> MGHHHHHHHHHHSSGHIEGRHMRVGYVSTNYSLGCKADKTIKLSSLSEERVLKVSSSNLLCLKNILEWNLKHEILFFRISSNTIPLASHPKFHVNWKDKLSHILGDIGDFIKENSIRISMHPGQYVVLNSVREEVVRSSIMELKYHADLLDSMGIEGKIQIHVGSSMNGKEESLNRFIENFRKLPSNISKRLVIENDDKVFSVKDCLWISERTGIPVIFD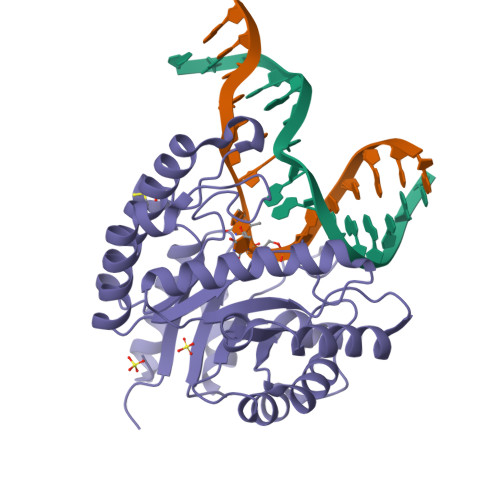NLHHSILNNGESLNDALSLVRRTWKDRPMIDYSEQEPGEKPGVHATTINEENFRRFVNEVDEVDIMLEVKDKEISALKAVKVLKELNKLD> KETAAAKFERQHMDSSTSAASSSN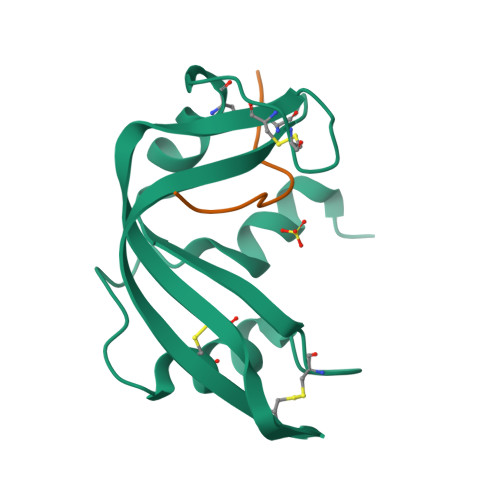YCNQMMKSRNLTKDRCKPVNTFVHESLADVQAVCSQKNVACKNGQTNCYQSYSTMSITDCRETGSSKYPNCAYKTTQANKHIIVACEGNPYVPV;> EGNPYVPVHFDASV> MANSLEPEPWFFKNLSRKDAERQLLAPGNTHGSFLIRESESTAGSFSLSVRDFDQNQGEVVKHYKIRNLDNGGFYISPRITFPGLHEL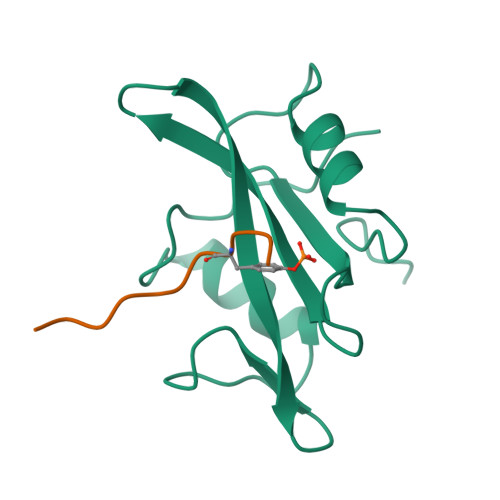VRHYTNASDGLCTRLSRPCQT;> EPQYEEIPIYL>[2x]MHHHHHHSSGRENLYFQGESTRRLILVGRTGAGKSATGNSILGQRRFFSRLGATSVTRACTTGSRRWDKC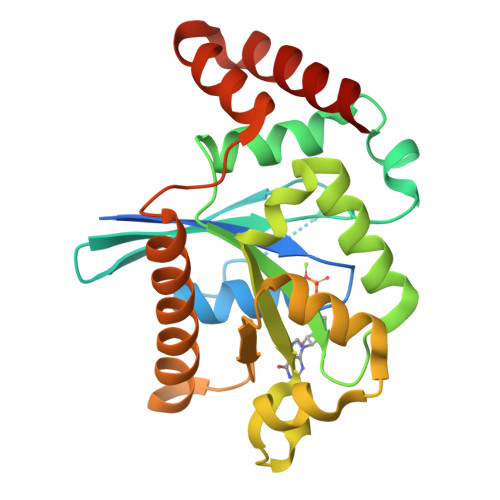HVEVVDTPDIFSSQVSKTDPGCEERGHCYLLSAPGPHALLLVTQLGRFTAQDQQAVRQVRDMFGEDVLKWMVIVFTRKEDLAGGSLHDYVSNTENRALRELVAECGGRVCAFDNRATGREQEAQVVQLLGMVEGLVLEHKGAHYSNEVYELAQVLRWAGPEERLRRVAERVAARVQR> MHHHHHHENLYFQSNAAKNSLTTKSLFK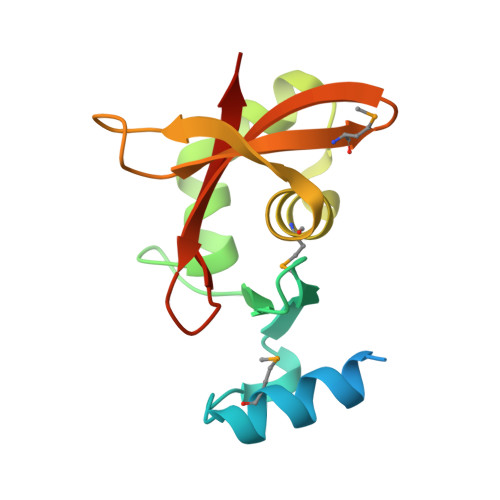EMTIQGIKFTPENVVGAAKDNSGKIIFLEKGNSKSGLQHIVEEHGDQFAQIGVSEARIPDVVMKAVTDGKIVGYQGAGAGRPIYETMIDGKKYNIAVTVGSNGYVVGANLRGSVK Replication initiator proteins (Reps) from the HUH-endonuclease superfamily process specific single-stranded DNA (ssDNA) sequences to initiate rolling circle/hairpin replication in viruses, such as crop ravaging geminiviruses and human disease causing parvoviruses. At the heart of DNA processing of all HUH-endonucleases is a structurally defined catalytic nickase domain that first recognizes a specific sequence/structure of DNA; nicks ssDNA at a ‘nic site’ to yield a sequestered 5′ end that remains covalently bound to the HUH endonuclease and a free 3′OH that can be used as a primer for DNA replication; and finally, facilitates a strand transfer reaction to resolve the covalent intermediate. To uncover the ssDNA recognition mechanism of Reps and identify potential motifs that might confer sequence specificity, we solved the first high resolution crystal structures of two Rep nickase domains from Porcine circovirus 2 (PCV2) and Wheat dwarf virus (WDV) with 12% sequence identity, bound to ssDNA encoding minimal sequences comprising the respective origin of replication (ori) sequences. With this, we term this turn-β-turn structural motif as the ‘single-stranded DNA Bridging Motif’ (sDBM), and suggest that it is the main binding moiety responsible for recognition and conformation priming of ssDNA by Rep HUH-endonucleases.

We present structures of two 10-mer bound structures of inactive PCV2Y96F (1.93 Å resolution) and WDVY106F (1.80 Å resolution), and one 8-mer bound WDVY106F (2.61 Å resolution) structure. The pre-cleavage state was captured by mutating the catalytic tyrosine to phenylalanine. All three structures are in complex with the divalent cofactor manganese. Additionally, the catalytic tyrosine (though a Phe mutant in the structures) is positioned for nucleophilic attack of the scissile phosphate, where the active oxygen of PCV2 and WDV is measured at 2.2 and 2.9 Å from the phosphate, respectively. The U-shaped DNA sits in a shallow channel on the surface of one face of the Rep protein with a distinct topological ‘nose’ that juts out in the center of the U. The bent conformation of the ssDNA in the Rep structures is driven by both intermolecular interactions with the topological ‘nose’ of the protein and by intramolecular Watson–Crick base pairing between T−4 and A+1 along with adjacent hydrogen bonding between N3 of T−1 and N3 of A−3. In the WDVY106F + 10-mer structure, residues His91 and Asp93 in this ‘bridging’ motif specifically contact the base of A−5, whereas Arg79 and His81 in the PCV2 structure contact the base of G−5. We hypothesize that these contacts play a major role in conferring specificity differences at the −5 position. His91 and Asn93 of WDV facilitate polar contacts with A−5, which may give WDV more specificity at position –5, whereas there is only one polar contact with G−5 by His82 in the PCV2 structure, which results in less stringent specificity.

> MASSSTPRFRVYSKYLFLTYPQCTLEPQYALDSLRTLLNKYEPLYIAAVRELHEDGSPHLHVLVQNKLRASITNPNALNLRMDTSPFSIFHPNIQAAKDCNQVRDFITKEVDSDVNTAEWGTFVAVSTPGRKDRDAD In the first step of the HP, GFAT synthesizes d-glucosamine-6-phosphate (GlcN6P) from l-glutamine (l-Gln) and Frc6P, releasing l-glutamate (l-Glu). GFAT contains two domains: the glutaminase domain responsible for releasing ammonia in the hydrolysis of l-Gln to l-Glu and the isomerase/transferase domain, which catalyzes both the isomerization of Frc6P to d-glucose-6-phosphate (Glc6P) as well as the transfer of ammonia to Glc6P to produce GlcN6P. The active sites of the two domains are linked by an ammonia channel, which forms when GFAT engages with both of its substrates, l-Gln and Frc6P. The main distinctive feature between prokaryotic and eukaryotic GFAT is the feedback inhibition by the HP product UDP-GlcNAc, which inhibits the glutaminase function.

As a negative control we generated a GFAT-1 variant that prevents UDP-GlcNAc binding by mutating Gly461, which is located at the bottom of the UDP-GlcNAc-binding pocket. Kinetic measurements showed that GFAT-1 G461E has similar kinetic properties like wild type GFAT-1 for l-Glu and d-GlcN6P synthesis. GFAT-1 G461E did not respond to UDP-GlcNAc treatment, as expected from the crystal structure.

>[2x]MCGIFAYLNYHVPRTRREILETLIKGLQRLEYRGYDSAGVGFDGGNDKDWEANACKIQLIKKKGKVKALDEEVHKQQDMDLDIEFDVHLGIAHTRWATHGEPSPVNSHPQRSDKNNEFIVIHNGIITNYKDLKKFLESKGYDFESETDTETIAKLVKYMYDNRESQDTSFTTLVERVIQQLEGAFALVFKSVHFPGQAVGTRRGSPLLIGVRSEHKLSTDHIPILYRTGKDKKGSCNLSRVDSTTCLFPVEEKAVEYYFASDASAVIEHTNRVIFLEDDDVAAVVDGRLSIHRIKRTAGHHHHHHDHPGRAVQTLQMELQQIMKGNFSSFMQKEIFEQPESVVNTMRGRVNFDDYTVNLGGLKDHIKEIQRCRRLILIACGTSYHAGVATRQVLEELTELPVMVELASDFLDRNTPVFRDDVCFFLSQSGETADTLMGLRYCKERGALTVGITNTVGSSISRETDCEVHINAGPEIGVASTKAYTSQFVSLVMFALMMCDDRISMQERRKEIMLGLKRLPDLIKEVLSMDDEIQKLATELYHQKSVLIMGRGYHYATCLEGALKIKEITYMHSEGILAGELKHGPLALVDKLMPVIMIIMRDHTYAKCQNALQQVVARQGRPVVICDKEDTETIKNTKRTIKVPHSVDCLQGILSVIPLQLLAFHLAVLRGYDVDFPRNLAKSVTVE>MSLKITEIETLRPEEFPNLLWVLVHTDEGITGLGETFYGACSAEAYIHEWAANRLIGEDPLQIDRHAKRLSGYLGFRSAGAEMRGNSALDIALWDIFGKATGQPIYQLLGGKCRDTIRTYNTCAGPHYVRTAKQQSVANWGLANSVSARYDDLNAFLHRADELALDLLDSGITAMKIWPFDPYAEASDGYYISKSDLKRALEPFEKIRRAVGDKMDVMVEFHSLWNLPPALQIAEALREYETFWHEDPIRMDSLSSLKRYAERSLAPVCASETLATRWGFRDLLETNAAGIVMLDISWCGGLSEARKIASMAEAWHLPVAPHDCTGPVVLTASTHLSLNAPNALVQESVRAFYDGWYRDLVTALPTVKDGHITVPDGPGLGLELMPDIRERLTIAV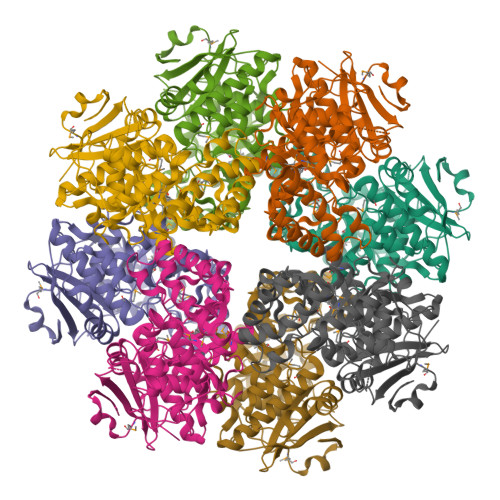RNTSDCEGHHHHHH[2x]>SMADLSSKRSRVVGVVVPLIHTNFADEIIKGLYETTISSGYELLITYLDEDEDHQYQVFQTLLSRQVGAVFMLSLDIPSWMIDKLLEEQISVI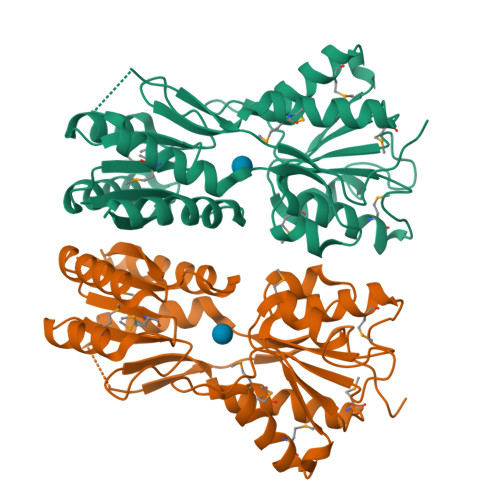SLTALLSEQISAVTSNEFEMMNSIVDYLIDMGHKNIALVGDTKLTTNISSTRRTNFIKSMTDHNLAYENIFLYGNDHSYETGYTSVTTGYDINQLPFTAAIATADMVGQGLINAMSDHGKTVPEDLSIVTIDGLQQTEIARPKLTTVKQDFPEIGRIAMQLFLDSDSEKTEPQIIYIPTELIQRDSVLNLNSTK[2x]>[2x]MATQLAPEVPQFTYHSSPTATEAFAAWLKDNPQAIPAHSHPWDVSRSDIYVEDRWQPIFAEMRAKAPVNRVPDSPYGAYWNVASHKAIMHVESLPELFSSSWQYGGITIGDPP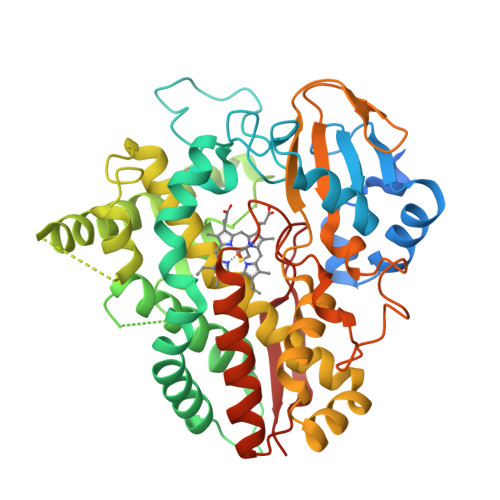EDVDPQKLAERQLPMFIAMDRPDHTGQRRTVAPAFTPAKMVEMEAEIRRRTASVLDSLPWGERFDWVDKVSIELTTGMLAILFGFPWADRRLLTFWSDWAGDVELTLARELADTRFGFLGEMAHYFQRLWGARMQAPPSGDLISMMIHSEAMNHMSPQEFMGNLVLLIVGGNDTTRNTMSGIVHALDKFPDQRELLERDASLIPNAVQECIRYVTPLAHMRRTATADTELFGNQIKAGEKVILWYISANRDETVFENPDKLMVDRPNARRHLSFGHGIHRCVGARLAELQLRILLEEMHERRMRVRVAGEVERVRANFVHGFRKLEVELEKR2,6-DIAMINO-8-(2-DIMETHYLAMINOETHYLSULFANYLMETHYL)-3H-QUINAZOLIN-4-ONE 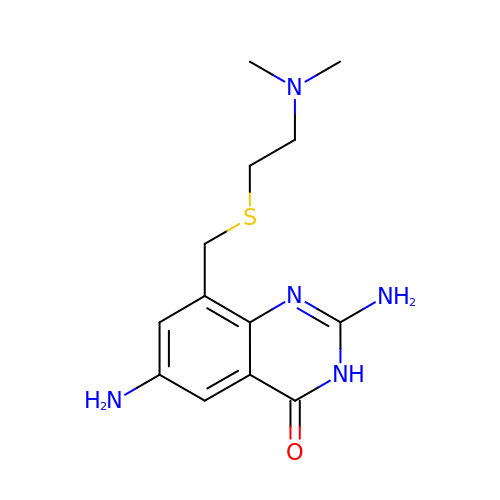| C13 H19 N5 O S | FDIXHXDLCOSDFY-UHFFFAOYSA-N The Escherichia coli enzyme EcAIII catalyzes the hydrolysis of L‐Asn to L‐Asp and ammonia. Using a nature‐inspired mutagenesis approach, we designed and produced five new EcAIII variants (M200I, M200L, M200K, M200T, M200W). The modified proteins were characterized by spectroscopic and crystallographic methods. All new variants were enzymatically active, confirming that the applied mutagenesis procedure has been successful.

The determined crystal structures revealed new conformational states of the EcAIII molecule carrying the M200W mutation and allowed a high‐resolution observation of an acyl‐enzyme intermediate with the M200L mutant.

>[2x]MGKAVIAIHGGAGAISRAQMSLQQELRYIEALSAIVETGQKMLEAGESALDVVTEAVRLLEECPLFNAGIGAVFTRDETHELDACVMDGNTLKAGAVAGVSHLRNPVLAARLVMEQSPHVMMIGEGAENFAFARGMERVSPEIFSTSLRYEQLLAARKEGATVLDHSGAPLDEKQKMG;>[2x]TVGAVALDLDGNLAAATSTGGWTNKLPGRVGDSPLVGAGCYANNASVAVSCTGTGEVFIRALAAYDIAALMDYGGLSLAEACERVVMEKLPALGGSGGLIAIDHEGNVALPFNTEGMYRAWGYAGDTPTTGIYREKGDTVATQ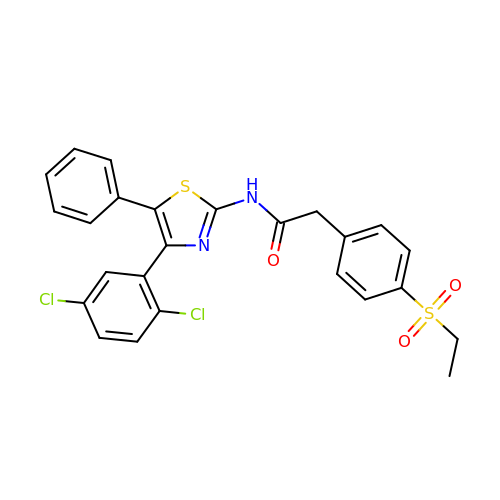N-[4-(2,5-dichlorophenyl)-5-phenyl-1,3-thiazol-2-yl]-2-[4-(ethylsulfonyl)phenyl]acetamide | C25 H20 Cl2 N2 O3 S2 | NUQYLKJMFVEWEU-UHFFFAOYSA-N> MPALPEDGGSGAFPPGHFKEPKRLYCKNGGFFL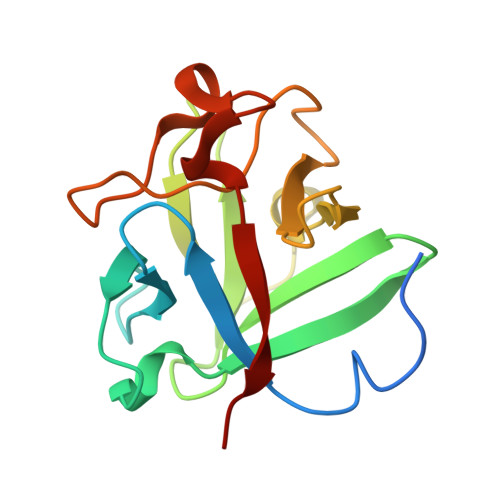RIHPDGRVDGVREKSDPHIKLQLQAEERGVVSIKGVLANRYLAMKEDGRLLASKIVTDECFFFERLESNNYNTYRSRKYTSWYVALKRTGQYKLGPKTGPGQKAILFLPMSAKS> GAMSHPHDSKVFPDLPEHQDNPSQLRLQHDGLATDDKARLEPMCLAEYLISGPGGMDPDIEIDDDTYDECREVLSRILEDAYTQSGTFRRLMNYAYDQELHDVEQRWLLGAGENFGTTVTDEDLESSEGRKVIALNLDDTDDDSIPEYYESNDGPQQFDTTRSFIHQVVHALTHLQDKEDSNPRGPVVEYTNIILKEM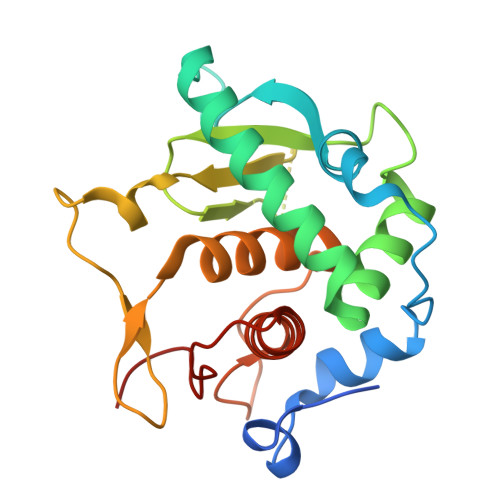GHTSPPRIAYEFSN>[12x]MAGPLSGLRVVELAGIGPGPHAAMILGDLGADVVRIDRPSSVDGISRDAMLRNRRIVTADLKSDQGLELALKLIAKADVLIEGYRPGVTERLGLGPEECAKVNDRLIYARMTGWGQTGPRSQQAGHDINYISLNGILHAIGRGDERPVPPLNLVGDFGGGSMFLLVGILAALW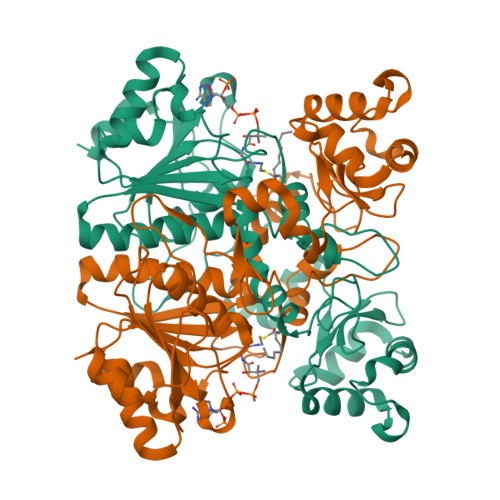ERQSSGKGQVVDAAMVDGSSVLIQMMWAMRATGMWTDTRGANMLDGGAPYYDTYECADGRYVAVGAIEPQFYAAMLAGLGLDAAELPPQNDRARWPELRALLTEAFASHDRDHWGAVFANSDACVTPVLAFGEVHNEPHIIERNTFYEANGGWQPMPAPRFSRTASSQPRPPAATIDIEAVLTDWDGGSGC ethyl (2Z,4S)-4-{[N-(3-cyclopropylpropanoyl)-L-phenylalanyl]amino}-5-[(3S)-2-oxopyrrolidin-3-yl]pent-2-enoate | C26 H35 N3 O5 | 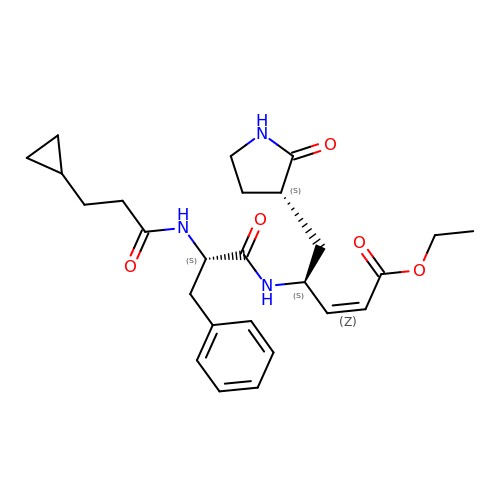QRJJXRNUFIJDHO-BDTNDASRSA-N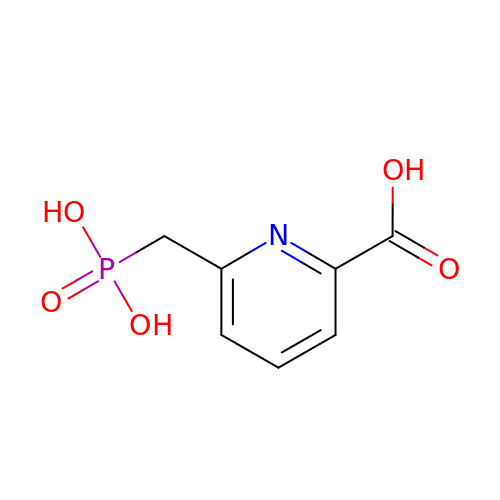6-(phosphonomethyl)pyridine-2-carboxylic acid | C7 H8 N O5 P | HIDJRVUSOKZHOS-UHFFFAOYSA-N> MDPKISEMHPALRLVDPQIQLAVTRMENAVGRDQNNVGPKVYPIILRLGSPLSLNMARKTLNSLEDKAFQLTPIAVQMTKLATTEELPDEFVVVTVK;> MAASKPVEAAVVAAAVPSSGSGVGGGGTAGPGTGGLPRWQLALAVGAPLLLGAGAIYLWSRQQRRREARGRGDASGLKRNSERKTPEGRASPAPGSGHPEGPGAHLDMNSLDRAQAAKNKGNKYFKAGKYEQAIQCYTEAISLCPTEKNVDLSTFYQNRAAAFEQLQKWKEVAQDCTKAVELNPKYVKALFRRAKAHEKLDNKKECLEDVTAVCILEGFQNQQSMLLADKVLKLLGKEKAKEKYKNREPLMPSPQFIKSYFSSFTDDIISQPMLKGEKSDEDKDKEGEALEVKENSGYLKAKQYMEEENYDKIISECSKEIDAEGKYMAEALLLRATFYLLIGNANAAKPDLDKVISLKEANVKLRANALIKRGSMYMQQQQPLLSTQDFNMAADIDPQNADVYHHRGQLKILLDQVEEAVADFDECIRLRPESALAQAQKCFALYRQAYTGNNSSQIQAAMKGFEEVIKKFPRCAEGYALYAQALTDQQQFGKADEMYDKCIDLEPDNATTYVHKGLLQLQWKQDLDRGLELISKAIEIDNKCDFAYETMGTIEVQRGNMEKAIDMFNKAINLAKSEMEMAHLYSLCDAAHAQTEVAKKYGLKPPTL

Orf9b is a unique accessory protein of SARS-CoV-2 and SARS-CoV. It is implicated in immune evasion by targeting mitochondria, where it associates with the versatile adapter TOM70. TOM70 is a multifunctional protein anchored to the mitochondrial outer membrane. It is a surface receptor of the translocase of the outer membrane (TOM) complex, the gateway of protein import in mitochondria.

We determined the crystal structure of the hTOM70 ΔN2/SARS-CoV-2 orf9b complex to 2.2 Å. One copy of TOM70 and one copy of orf9b are present in the asymmetric unit, consistent with our stoichiometry assessment. While the majority of hTOM70 residues were visible in our final structure, we found a central portion of SARS-CoV-2 orf9b (residues 43-78) was bound to hTOM70, but the remnant of orf9b was disordered. The visible portion of SARS-CoV-2 orf9b adopts a helical conformation: The N-terminal region of the fragment folds into a “U-turn” shaped loop that is followed by a long, slightly bent helix and a short helix; the C-terminal region of the fragment extends towards the proximity of hTOM70 NTD. This is in stark contrast to the β-sheet-rich conformation adopted by the same fragment in the orf9b homodimer. Using PISA software, we calculated the buried interface area between hTOM70 and SARS-CoV-2 orf9b of ~2000 Å2 and the solvation free energy gain (ΔiG) of −33.8 kcal/M. Owing to the high resolution of this structure, we were able to identify extensive interactions between the two proteins: (1) Polar contacts include 12 potential hydrogen bonds and 7 potential salt bridges, involving 10 residues of hTOM70 (from α13, α19, α21, α23, and α25 helices) and 11 residues of SARS-CoV-2 orf9b. Of note, multiple salt bridges (distance 2.7–3.3 Å) were identified between E549, H583 of hTOM70, and R58, E65 of orf9b, suggesting their importance in the interaction. (2) We identified 23 non-polar residues on the surface of the CTD pocket interacting with SARS-CoV-2 orf9b. Comparing the structure of hTOM70/orf9b complex and the unliganded structures indicates that the binding of orf9b induces evident conformational changes, which includes movement of the bridging helix outward or downward compared with the corresponding helix in yeast TOM70 or TOM71 structure, and the bottom helix is pressed down by the N-terminal portion of the orf9b. Collectively, we identified a highly flexible region of the CTD-pocket of hTOM70 associated with orf9b binding. By occupying the CTD pocket, the orf9b may lock the conformation of hTOM70 into a rigid state.>[2x]ACAUGC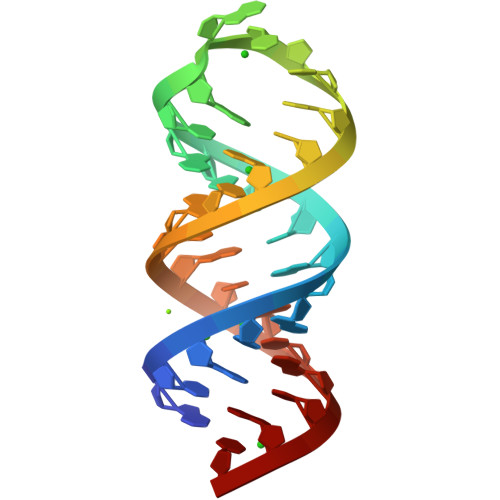ACAUGCAAUUUGUGUAUGUGUAUGU6-CHLORO-2-FLUOROPURINE | C5 H2 Cl F N4 | 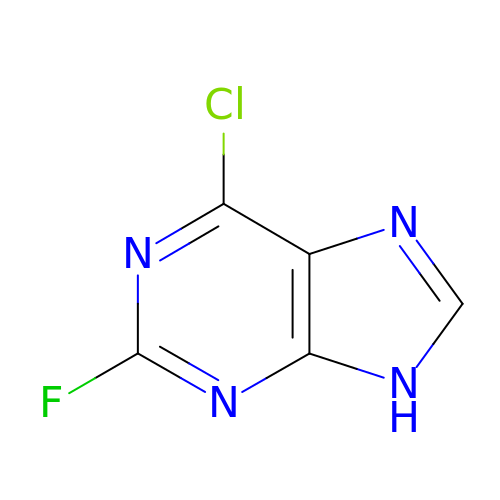UNRIYCIDCQDGQE-UHFFFAOYSA-N>[4x]SKDRMVELLQEHFELNLYEARAYVALVAFGVLTPAELASVSEVPAPRTYDVLRSLEKKGFAMTQPGKTNKYRPVHPANVLEKFIQDWQERVKEELEAKKKAKEELLELMAPLIETEVPKYGVERVWVVRGIKNSTLKTKEMLEEAQNEILLADDGFIAVN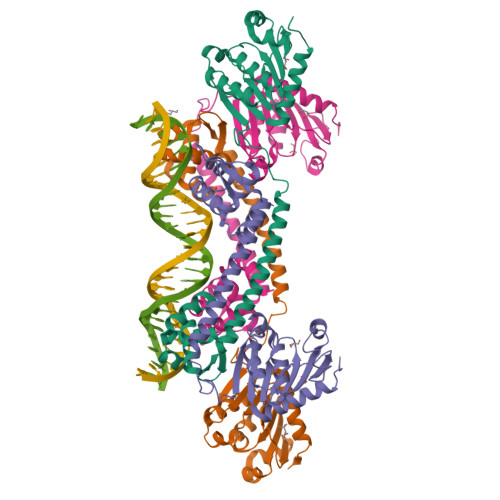LEDDIIKAVDRGVKTKILLTKNLLPRLKASKIIDYAKEGKLELRALDKFDLPMLICDEEVFFALEDLAARYFNYETQVWIKDHRVVALFKEKFNEYWEKAEKV>MESLLNRLYDALGLDAPEDEPLLIIDDGIQVYFNESDHTLEMCCPFMPLPDDILTLQHFLRLNYTSAVTIGADADNTALVALYRLPQTSTEEEALTGFELFISNVK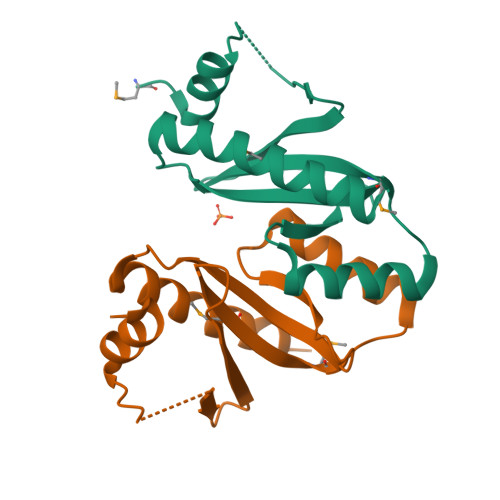QLKEHYA[2x]LapD is a c-di-GMP receptor that translates changes in the concentration of this cytosolic second messenger into cell-surface events via an inside-out signaling mechanism that ultimately controls cell adhesion. Specifically, c-di-GMP-bound LapD engages the periplasmic protease LapG through its Per-Arnt-Sim (PAS)-like domain, preventing it from cleaving the cell surface-bound large adhesin LapA, a protein mediating cell adhesion to multiple substrates. In contrast, c-di-GMP-unbound LapD adopts an autoinhibited conformation and loses its affinity for LapG. To address these shortcomings, we report here two structures, that of the output domain of a LapD ortholog from L. pneumophila, also known and referred to here as CdgS9, and that of LapG in complex with the same output domain.

While the homogeneous complexes failed to crystallize thus far despite the best of our efforts, we were successful in determining the structure of L. pneumophila CdgS9Output bound to P. fluorescens LapG (see details in ‘Materials and methods’). The crystallized complex consists of two CdgS9 output domain molecules that adopt a similar parallel dimer conformation as in the apo-CdgS9Output structure. The output domain dimer is bound to one LapG molecule at a lateral docking site, with an interaction surface of 1290 Å2 (with a calculated ΔGint = −16.3 kcal/mol; PISA [Krissinel and Henrick, 2007]) and involving both molecules of the CdgS9Output dimer to a similar extent. As predicted by the biochemical analysis, the conserved tryptophan residue (W126) is the major anchor point on CdgS9 as it inserts into a hydrophobic pocket at the bottom of LapG. While there are contributions from a limited number of hydrogen bonds and a water-mediated interaction, the interface appears to be dominated by hydrophobic contacts and shape-complementarity of the interacting elements. The resulting complex is asymmetric with regard to the output domain dimer, manifested by a 5 Å tilt and vertical offset of one PAS domain fold relative to the other. The central helices α1 are pushed closer together—a movement permitted by smaller residues at the interface (S48 and S52), a perpendicular-to-parallel stacking transition of one of the F33–F34 residue pairs, and the relocation of R75 from the dimer interface to a more surface-exposed position. The net result is a transition from a four-helix bundle with poor shape complementarity with LapG to a two-helix bundle and an overall shape that is able to accommodate LapG. First, we identified a rare di-calcium binding motif in the N-terminal lobe of P. fluorescens LapG, which is in contrast to the single calcium ion bound at the same site in the L. pneumophila LapG structure.

>TYFITMNNARNFFIQQLESNAQDTATSLGLSLSQSLINHDVPTMDSMVKAVFDRGYFSSIKVQDIKGKVIILKKQLPQESDIPQWFVNLIKWPSTEKSSLIMDGWMQAGVVLVASDPSYVYASLWRNAVEM[4x];>ADWDFSAISRKATALYGPLGAGQQRIDAWQNLLATQKQVSEMEKLKVVNLFFNKQMRYVEDIDLWHEVDYWETPIEALWKGAGDCEDYAIAKYFSLRHLGVASDKLRITYVKALRQNRAHMVLTYYSSPDAMPLVLDSLIDPIKPAAERTDLLPVYSFNAEGLYLPGAKGNKKVGDTKRLSRWQDVLKKMQAEGFPV[2x]> GAMASGKVVKFSYMWTINNFSFCREEMGEVIKSSTFSSGANDKLKWCLRVNPKGLDEESKDYLSLYLLLVSCPKSEVRAKFKFSILNAK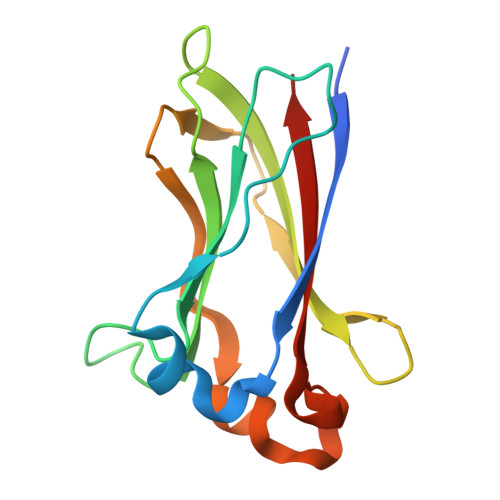GEETKAMESQRAYRFVQGKDWGFKKFIRRDFLLDEANGLLPDDKLTLFCEVSVVQD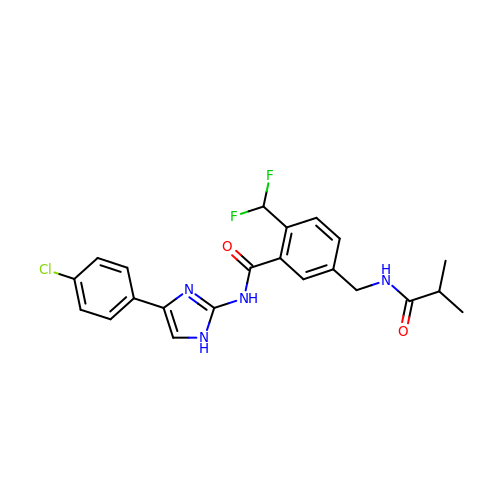N-[4-(4-chlorophenyl)-1H-imidazol-2-yl]-2-(difluoromethyl)-5-{[(2-methylpropanoyl)amino]methyl}benzamide | C22 H21 Cl F2 N4 O2 | WMRBMFOTNQIZHQ-UHFFFAOYSA-N> XSLSDKDKAAVKLLWSKISKSSDAIGNDALSRMIVVYPQTKTYFAHWPDLSPGSPHVKAHGKTVMGGIALAVSKIDDLRAGLLDLSEQHAYKLRVDPANFKILSHCILVVISMMFPKEFTPEAHVSLDKFLSGVSLALSE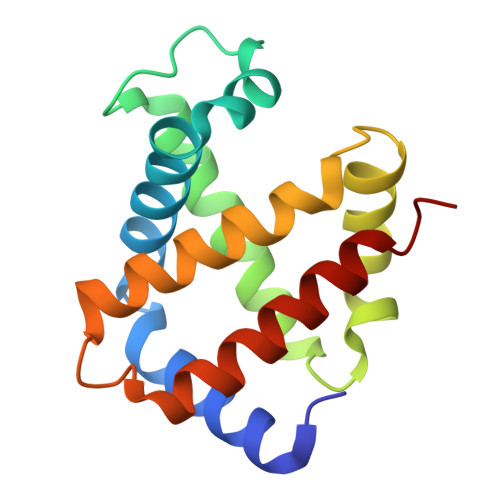RYR>MNRLPSSASALACSAHALNLIEKRTLDHEEMKALNREVIEYFKEHVNPGFLEYRKSVTAGGDYGAVEWQAGSLNTLVDTQGQEFIDCLGGFGIFNVGHRNPVVVSAVQNQLAKQPLHSQELLDPLRAMLAKTLAALTPGKLKYSFFCNSGTESVEAALKLAKAYQSPRGKFTFIATSGAFHGKSLGALSATAKSTFRKPFMPLLPGFRHVPFGNIEAMRTALNECKKTGDDVAAVILEPIQGEGGVILPPPGYLTAVRK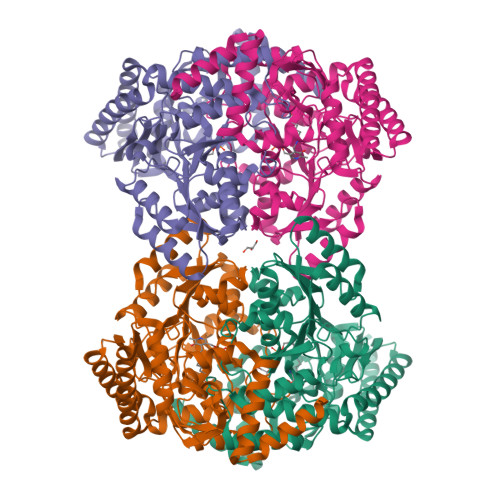LCDEFGALMILDEVQTGMGRTGKMFACEHENVQPDILCLAKALGGGVMPIGATIATEEVFSVLFDNPFLHTTTFGGNPLACAAALATINVLLEQNLPAQAEQKGDMLLDGFRQLAREYPDLVQEARGKGMLMAIEFVDNEIGYNFASEMFRQRVLVAGTLNNAKTIRIEPPLTLTIEQCELVIKAARKALAAMRVSVEEALEHHHHHH[4x]>CWTYEEEYYFRSNFLQQYNKDIRPLNDLSKPISVGIHLEIAKMNDFNLAEGRLKIQTYLILQWYDEKIFWNESTYPIPKLMVSSKKIWSPAISVYYTENEMDSKDQFQMEIYKNGSVHQWKSFYFNILCDVNARAFPFDKYTCETMFYFNDYDIQTAIFSSFRCISSTDLSRKAWYVSFSCDTKIGEEGSLGQLSLKLVRKVSLQCLSVLLPLFIFFILNIMIGYLPIESGEKVTFATTVFLSNVIYIDNLSKQLPKESSEIPLIFLCHIFLAFLSGLSAVGTIITSKIFCKYKSTESAPSPSPAPANNKIDVKKNSQIYSISKEGRVEKEANSSDG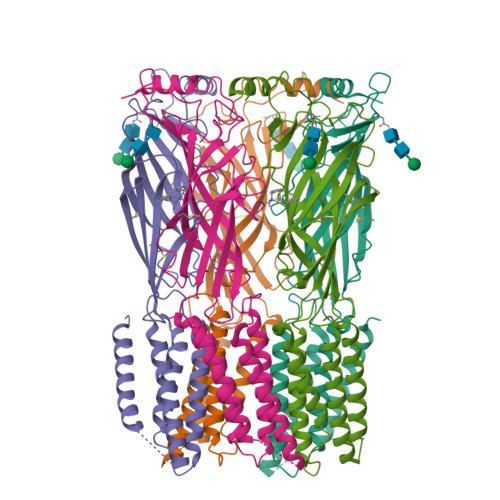IKATTTTTTTTITEDLKKICLSYAKIESAILYIMTFISILCALVFTSLFFESFLD[5x]A deazaflavin-dependent nitroreductase (Ddn) from Mycobacterium tuberculosis catalyzes the reduction of nitroimidazoles such as PA-824, resulting in intracellular release of lethal reactive nitrogen species. The N-terminal 30 residues of Ddn are functionally important but are flexible or access multiple conformations, preventing structural characterization of the full-length, enzymatically active enzyme. The split barrel-like fold is characterized by a central six-stranded antiparallel β barrel in a Greek key topology with four α helices: A at the N terminus (the putative helix removed for Ddn structure determination), B after an extended loop between strands β3 and β4, and C and D between strands β5 and β6. The identification of these residues and the lack of classic catalytic residues in the active site suggest that Ddn functions primarily by precisely orienting PA-824 for efficient direct hydride transfer from F420 and potentially through additional transition-state stabilization.

Deletion of 26–50 residues from the N terminus showed high levels of soluble protein expression, and removal of 30, 33, or 40 residues produced nonaggregated monomeric protein. As expected (Manjunatha et al., 2006a; Taylor et al., 2010), the backbone trace shows high similarity to proteins in the split barrel-like family of flavin-binding proteins. The initial structure was then used to solve the structure of the longer NΔ30 construct by molecular replacement based on a 1.55 Å data set (Apo-1 in Table 1) and of a 1.85 Å resolution NΔ33 crystal (P3221 space group; Apo-2 in Table 1). All but the first five amino-terminal residues could be built into the electron density for both crystal forms (36–151 and 39–151, respectively). The asymmetric units (ASUs) for the Apo-1 and Apo-2 crystals both contain single molecules with similar structures (root-mean-square deviation [rmsd] is 0.96 Å). This alignment omits 14 of 113 shared Cα atoms because of conformational differences in the same regions that differ upon coenzyme binding. In Apo-1 and Apo-2, α helix D is highly disrupted, with repositioning of residues 129–144 relative to the holo-enzyme structures complementing movement of the post-β3 loop. In Apo-2, this helix stops at Y136 and instead a helix forms upstream from residues 139–143, and residues 136–143 display higher ADPs.

> GEGLGGTFQKIPVALLTTTGRKTGQPRVNPLYFLRDGGRVIVAASKGGAEKNPMWYLNLKANPKVQVQIKKEVLDLTARDATDEERAEYWPQLVTMYPSYQDYQSWTDRTIPIVVCEP> SPNSQYLKTRILDIYTPEQRAGIEKSEDWRQFSRRMHTHFPKLMNELDSVYGNNEALLPMLEMLLAQAWQSYSQRNSSLKDIDIARENNPDWILSNKQVGGVCYVDLFAGDLKGLKDKIPYFQELGLTYLHLMPLFKCPEGKSDGGYAVSSYRDVNPALGTIGDLREVIAALHEAGISAVVDFIFNHTSNEHEWAQRCAAGDPLFDNFYYIFPDRRMPDQYDRTLREIFPDQHPGGFSQLEDGRWVWTTFNSFQWDLNYSNPWVFRAMAGEMLFLANLGVDILRMDAVAFIWKQMGTSCENLPQAHALIRAFNAVMRIAAPAVFFKSEAIDHPDQVVQYIGQDECQIGYNPLQMALLWNTLATREVNLLHQALTYRHNLPEHTAWVNYVRSHDDIGWTFADEDAAYLGISGYDHRQFLNRFFVNRFDGSFARGVPFQYNPS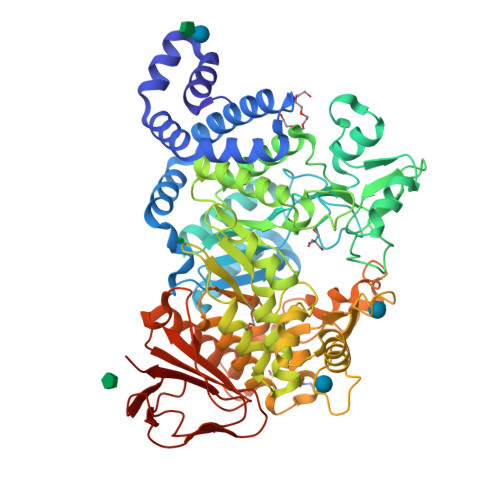TGDCRVSGTAAALVGLAQDDPHAVDRIKLLYSIALSTGGLPLIYLGDEVGTLNDDDWSQDSNKSDDSRWAHRPRYNEALYAQRNNPSTAAGQIYQDLRHMIAVRQSNPRFDGGRLVTFNTNNKHIIGYIRNNALLAFGNFSEYPQTVTAHTLQAMPFKAHDLIGGKTISLNQDLTLQPYQVMWLEIA> MVEAIVEFDYQAQHDDELTISVGEIITNIRKEDGGWWEGQINGRRG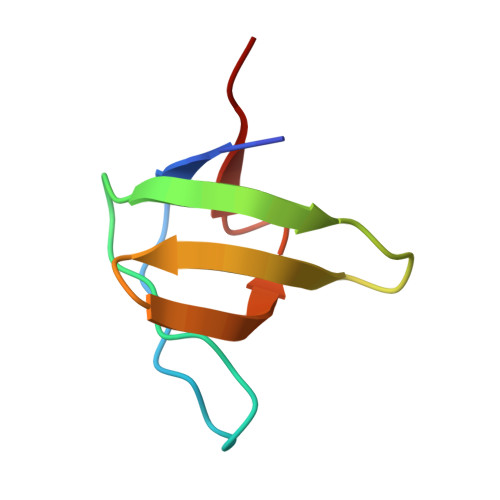LFPDNFVREIKK>PAMSNVPHKSSLPEGIRPGTVLRIRGLVPPNASRFHVNLLCGEEQGSDAALHFNPRLDTSEVVFNSKEQGSWGREERGPGVPFQRGQPFEVLIIASDDGFKAVVGDAQYHHFRHRLPLARVRLVEVGGDVQLDSVRIF[2x]

Galectins are members of the carbohydrate-binding lectin family with specificity for β-galactosides. The CRD is about 130 amino acids long, and the β-galactoside binding site is conserved among galectins, while differences both in adjacent β-strands and loop regions explain the variation in oligosaccharide binding affinity. Human galectin-7 (hGal-7) is a 15 kDa prototype galectin with a single CRD, monomeric but capable of dimerization in solution. Consequently galectin-7 has shown major roles in cancer development, by helping either in the elimination of certain tumour types or in the growth stimulation of others.

The high resolution (1.4 Å) structure gives an accurate insight into the molecular architecture of the protein with 99.3% of residues in the favoured Ramachandran plot area and 336 water molecules observed. The overall ‘jelly-roll’ fold is conserved compared with the previously obtained native and carbohydrate-bound complex structures. The two molecules in the asymmetric unit have similar overall characteristics (rmsd of 0.73 Å for all atoms) with little differences observed in some previously disordered regions. At the N-termini in particular molecule B presented some residual amino acids from the histidine-tag cleavage forming a tail lodging itself between two crystal-related symmetry molecules. Compared with the available structure, residues 1–3 were well ordered in both chains as well as Pro10 and Glu11. The CRD itself remains unchanged despite a slight movement in the adjacent loop composed of Arg74 and Gly75. Six residues showed potential alternate side chain conformation, namely Val18, Leu89, Asp95, Arg110, Arg117 and Arg133. Molecule A had an unusual difference electron density around the buried thiol group (Cys38), which is not conserved among galectins. Cysteine was replaced with an S-oxy cysteine in the structure, with potential oxidation due to radiation damage.> GANDTGRRILLNCDMGESFGAWRMGDDVHSMPLVDQANLACGFHAGD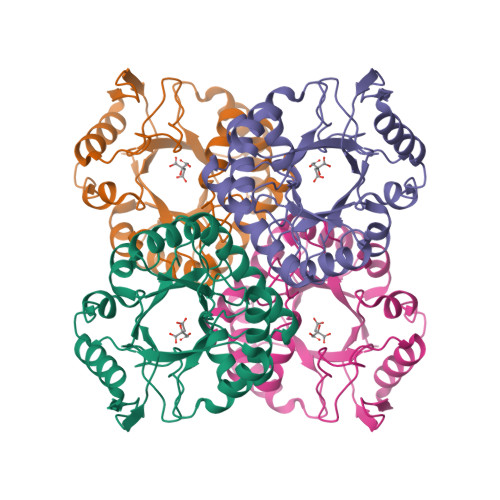PLTMRRAVELAVRHGVSIGAHPAYPDLSGFGRRSLACSAEEVHAMVLYQIGALDAFCRSLGTQVAYVKPHGALYNDLVGDDELLRAVLDACAAYRKGLPLMVLALADNGRELELADEADVPLLFEAFADRAYLPDGRLAPRRLGGAVHHDPQRIIEQALAIARGEAFPDYDGNPLRLTADSLCVHGDNPQSLAVLRRLRAALDSL> PTHIAICLYYKLGETPLPLVIETGKDAKALQIIKLAELYDIPVIED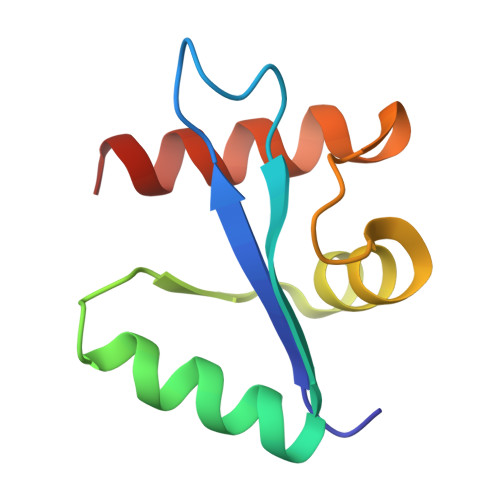IPLARSLYKNIHKGQYITEDFFEPVAQLIRIAIDLDY> EVHSRGQFIEQPNSVECDFTKLLSGTPPQVYNFNRLVFTNCNYNLTKLLSLFMVNEFSCDGISPDAIARGCYSSLTVDYFAYP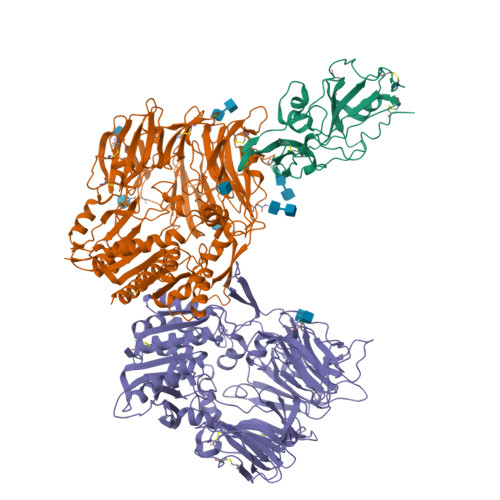LSMKSYMQPGSAGVISQYNYKQSFANPTCRIFATAPANLTITKPSSYSFISKCSRLTGDNSHIETPIVINPGEYSICKNFAPNGFSQDGDYFTRQLSQLEGGGILVGVGSVTPMTDTLQMGFIISVQYGTDTNSVCPMMD;>[2x]RKTYTLTDYLKNTYRLKLYSLRWISDHEYLYKQENNILVFNAEYGNSSVFLENSTFDEFGHSINDYSISPDGQFILLEYNYVKQWRHSYTASYDIYDLNKRQLITEERIPNNTQWVTWSPVGHKLAYVWNNDIYVKIEPNLPSYRITWTGKEDIIYNGITDWVYEEEVFSAYSALWWSPNGTFLAYAQFNDTEVPLIEYSFYSDESLQYPKTVRVPYPKAGAVNPTVKFFVVNTDSLSSVTNATSIQITAPASMLIGDHYLCDVTWATQERISLQWLRRIQNYSVMDICDYDESSGRWNCLVARQHIEMSTTGWVGRFRPSEPHFTLDGNSFYKIISNEEGYRHICYFQIDKKDCTFITKGTWEVIGIEALTSDYLYYISNEYKGMPGGRNLYKIQLSDYTKVTCLSCELNPERCQYYSVSFSKEAKYYQLRCSGPGLPLYTLHSSVNDKGLRVLEDNSALDKMLQNVQMPSKKLDFIILNETKFWYQMILPPHFDKSKKYPLLLDVYAGPCSQKADTVFRLNWATYLASTENIIVASFDGRGSGYQGDKIMHAINRRLGTFEVEDQIEAARQFSKMGFVDNKRIAIWGWSYGGYVTSMVLGSGSGVFKCGIAVAPVSRWEYYDSVYTERYMGLPTPEDNLDHYRNSTVMSRAENFKQVEYLLIHGTADDNVHFQQSAQISKALVDVGVDFQAMWYTDEDHGIASSTAHQHIYTHMSHFIKQCFSLP> MEVCLPNGHQIVDLINNAFEGRVSIYSAQEGWDKTISAQPDMMVCGGAVVCMHCLGVVGSLQRKLKHLPHHRCNQQIRHQDYVDVQFADRVTAHWKRGMLSFVCQMHAMMNDVSPEDLDRVRTEGGSLVELNWLQVDPNSMFRSIHSSWTDPLQVVDDLDTKLDQYWTALNLMIDSSDLVPNFMMRDPSHAFNGVRLEGDARQTQFSRTFDSRSSLEWGVMVYDYSE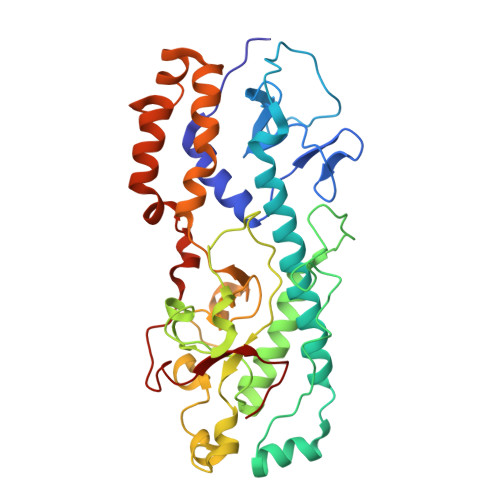LEHDPSKGRAYRKELVTPARDFGHFGLSHYSRATTPILGKMPAVFSGMLTGNCKMYPFIKGTAKLKTVRKLVDSVNHAWGVEKIRYALGPGGMTGWYNRTMQQAPIVLTPAALTMFSDTTKFGDLDYPVMIGDPMILG> MTATSDLIESLISYSWDDWQVTRQEARRVIAAIRNDNVPDATIAALDKSGSLIKLFQRVGPPELARSLIASIAGRTTMQRYQARNALIRSLINNPLGTQTDNW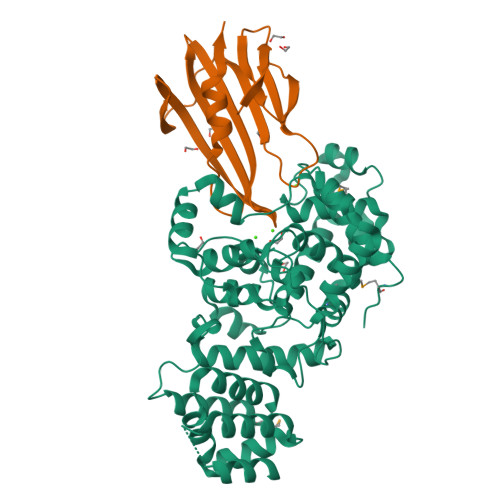IYFPTITFFDICADLADAAGRLGFAAAGATGVASQAIQGPFSGVGATGVNPTDLPSIAFGDQLKLLNKDPATVTKYSNPLGDLGAYLSQLSPQDKLNQAQTLVGQPISTLFPDAYPGNPPSRAKVMSAAARKYDLTPQLIGAIILAEQRDQTRDEDAKDYQAAVSIKSANTSIGLGQVVVSTAIKYELFTDLLGQPVRRGLSRKAVATLLASDEFNIFATARYIRYVANLASQQDLRKLPKTRGAFPSIDLRAYAGNPRNWPRDNVRALASEYTSRPWDDNLSPGWPMFVDDAYATFLDPGMRFPLEHHHHHH;> MKTVALILASLALLACTAESGVDFDKTLTHPNGLVVERPVGFDARRSAEGFRFDEGGKLRNPRQLEVQRQDAPPPPDLASRRLGDGEARYKVEEDDGGSAGSEYRLWAAKPAGARWIVVSASEQSEDGEPTFALAWALLERARLQLEHHHHHH> ETDEEPEEPGRRGSFVEMVDNLRGKSGQGYYVEMTVGSPPQTLNILVDTGSSNFAVGAAPHPFLHRYYQRQLSSTYRDLRKGVYVPYTQGKWEGELGTDLVSIPHGPNVTVRANIAAITESDKFFINGSNWEGILGLAYAEIARPDDSLEPFFDSLVKQTHVPNLFSLQLCGAGFPLNQSEVLASVGGSMIIGGIDHSLYTGSLWYTPIRREWYYEVIIVRVEIN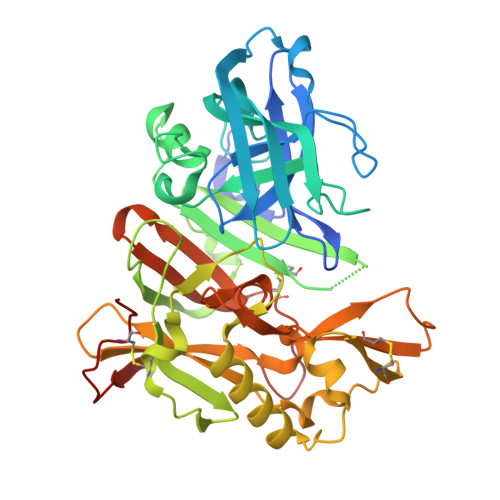GQDLKMDCKEYNYDKSIVDSGTTNLRLPKKVFEAAVASIKAASSTEKFPDGFWLGEQLVCWQAGTTPWNIFPVISLYLMGEVTNQSFRITILPQQYLRPVEDVATSQDDCYKFAISQSSTGTVMGAVIMEGFYVVFDRARKRIGFAVSACHVHDEFRTAAVEGPFVTLDMEDCGYNIPQTDEST>[2x]MGSDKIHHHHHHMKRFVETDKAPKAIGPYSQAVVVGNMMFVSGQIPIDPETGELVQGTIEEKTERVLENLKAILEAGGFSLKDVVKVTVFTTSMDYFQRVNE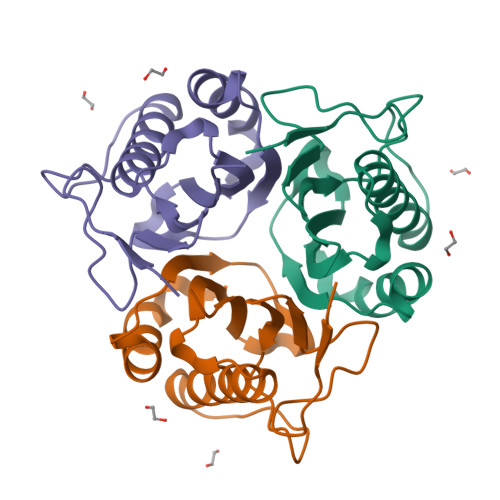VYSRYFGDHRPARSFVAVAQLPRNVEIEIEAIAVKEGE>MPVPNPTMPVKGAGTTLWVYKGSGDPYANPLSDVDWSRLAKVKDLTPGELTAESYDDSYLDDEDADWTATGQGQKSAGDTSFTLAWMPGEQGQQALLAWFNEGDTRAYKIRFPNGTVDVFRGWVSSIGKAVTAKEVITRTVKVTNVGRPSMAEDRSTVTAATGMTVTPASTSVVKGQSTTLTVAFQPEGVTDKSFRAVSADKTKATVSVSGMTITVNG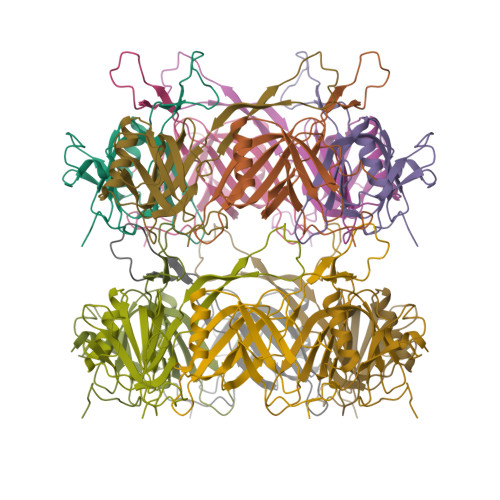VAAGKVNIPVVSGNGEFAAVAEITVTAS[12x]>[2x]SRAPYSGPQDLAALLEQIGCLKYLQVFEEQDVDLRIFLTLTESDLKEIGITAFGPKRKMTSAIARWHSSAR

Recent work has revealed that ANKS6 interacts with a related protein called ANKS3. Both ANKS6 and ANKS3 have a similar domain structure, with ankyrin repeats at the N-terminus and a SAM domain at the C-terminus. SAM domains consist of approximately 70 amino acids and adopt a globular structure generally containing a core of five α-helices. The protein-protein interactions of SAM domains are typically mediated by two distinct surfaces on the domain, termed the mid-loop (ML) and end-helix (EH) surfaces. Here we define the ANKS6/ANKS3 interaction by discovering that the ANKS6 SAM domain binds to the SAM domain of ANKS3.

Because the wild-type SAM domain is relatively insoluble, forming heterogeneous polymers, it cannot be crystallized directly. We therefore used a strategy that has proven successful for a number of other SAM domain polymers, where we attempt to crystallize SAM domains with mutations in the polymer interface. We were able to obtain a crystal structure of the L52A mutant. ANKS3-SAM L52A crystallized in space group P41 with two molecules in the asymmetric unit and the structure was solved to 1.6 Å resolution. Each SAM domain has the characteristic five α-helical fold and chains in the asymmetric unit are nearly identical (RMSD of 0.29 Å on backbone atoms and 0.3 Å on all atoms). Examination of the crystal packing reveals a triple helix of intertwined SAM polymers. Individual SAM polymers contain 8 SAMs per helical repeat, with each helical repeat measuring 72 Å in diameter and 100 Å in length. As expected from the mutational studies described above, the ANKS3 SAM domains associate via sequential interactions of ML and EH surfaces. The ML-surface, formed by residues spanning loop 2 through helix 4, is composed of a shallow hydrophobic patch (residues V32, I36, L40, and I48) flanked by negatively charged residues (D31, D33, D44, E47). The EH-surface encompasses the N-terminal portion of helix 5 and contains a critical Phe (F53) which packs against the hydrophobic patch of a neighboring ML-surface.> MGGKMEKITCVGHTALDYIFNVEKFPEPNTSIQIPSARKYYGGAAANTAVGIKKLGVNSELLSCVGYDFKNSGYERYLKNLDINISKLYYSEEEETPKAWIFTDKDNNQITFFLWGAAKHYKELNPPNFNTEIVHIATGDPEFNLKCAKKAYGNNLVSFDPGQDLPQYSKEM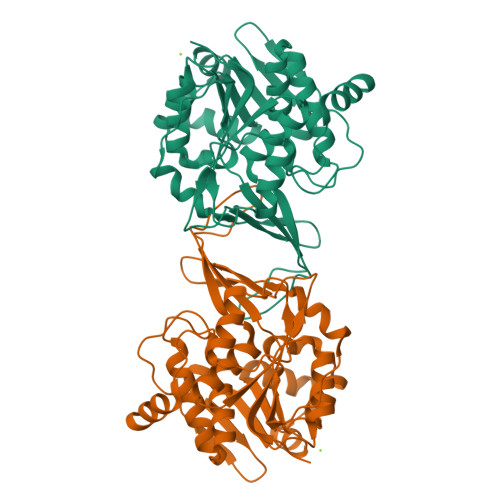LLEIIEHTNFLFMNKHEFERASNLLNFEIDDYLERVDALIVTKGSKGSVIYTKDKKIEIPCIKAGKVIDPTGAGDSYRAGFLSAYVKGYDLEKCGLIGAATASFVVEAKGCQTNLPTWDKVVERLEKHRI>[4x]MTDSSSLRGVDADTEKRINVGKKHLQTLRNLETRCHDSLQALVVIDAGSSSTRTNVFLAKTRSCPNKGRSIDPDSIQLIGAGKRFAGLRVVLEEWLDTYAGKDWESRPVDARLLFQYVPQMHEGAKKLMQLLEEDTVAILDSQLNEKQKVQVKALGIPVMLCSTAGVRDFHEWYRDALFVLLRHLINNPSPAHGYKFFTNPFWTRPITGAEEGLFAFITLNHLSRRLGEDPARSMIDEYGVKQSRNDLAGVVEVGGASAQIVFPLQEGTVLPSSVRAVNLQRERLLPERYPSADVVSVSFMQLGMASSAGLFLKELCSNDEFLQGGICSNPCLFKGFQQSCSAG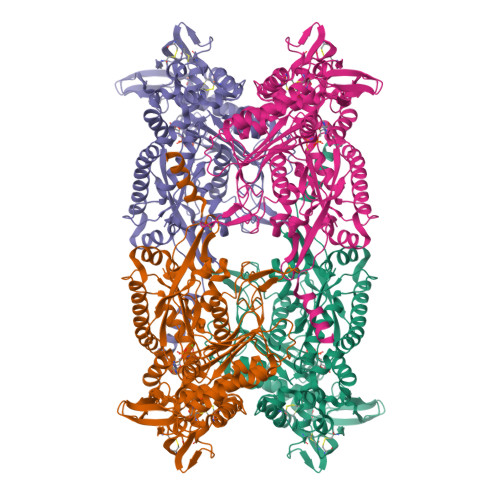EVEVRPDGSASVNEDVRKNRLKPLATYCSVNNPEISFKVTNEMQCRENSIDPTKPLAERMKIENCSIIKGTGNFDKCVSQVESILVAPKLPLPANIEAASSGFESVDQVFRFASSTAPMIVTGGGMLAAINTLKDHRLLRSDFSGDVEELAEAAREFCSSEVIIRTDGPVIQLPNARGEQKLNSLNFDLCKTMALTVSLLRHMAAGENQPSFIKWEKSIAGPDGKPLADLGWQVGVILHHVLFTEEWGRNAYEAGYSHNLEHHHHHH>MSAERILVTGGAGFIGSHLVDALLAKGYAVRVLDDLSTGKVGNLPMGDAGLELLVGDAADAALLADAVQGCDAVVHLAAVASVQASVEDPVATHQSNFIATLRLCEAMTAAGIRRVVFASAAAVYGNNGEGTPIAEDTPKSPLTPFAADKLASEYYLDFYRRQHGLEPVILRFFNIFGPRQDPSSPYSGVISIFSERAKAGRPITLFGDGGQTRDFVYVADLVKILVQGLESPAPAADATNVGLGGVTTLNDLIGALQQISGKPLQVSHGATRSGD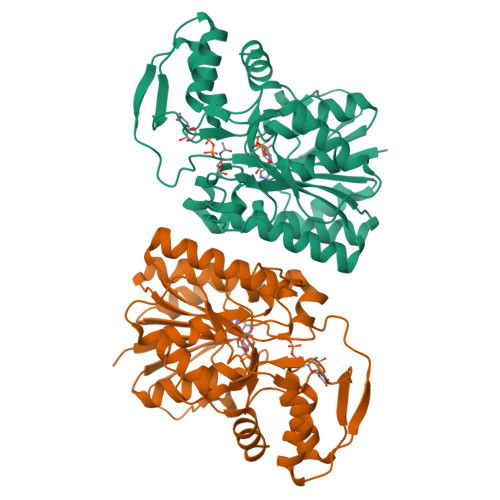IRHSKADNRRLRERFDLGTPSSLAEGLERLYRSL[2x]>[2x]GPDDYVPSQIAVNTSTLPGVVIGPADAHTYPRVIGELAGTSNQYVFNGGAIALMRGKFTPALPKIGSITYTFHQGN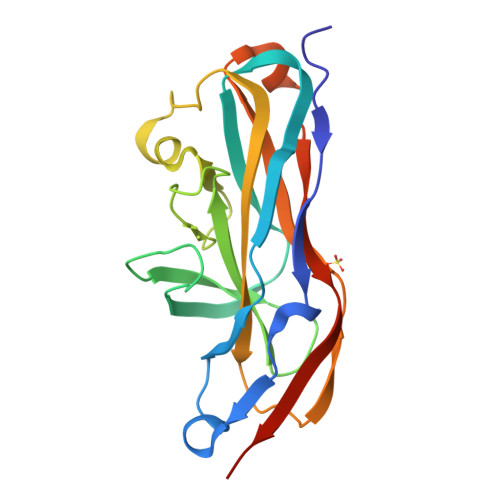SRDSSDFDIYDIGVSGLGIIIGMAGYWPATPLVPINSSGIYIDPVGANTNPNTYNGATASFGARLFVAFVATGRLPNGYITIPTRQLGTILLEAKRTSLNNKGLTAPVMLNGGRIQVQSQTHHHHHH CPS secretion is mediated by an ABC transporter containing KpsT and KpsM as its nucleotide-binding domain (NBD) and transmembrane domain, respectively. The transporter partners with the periplasmic and inner-membrane-anchored KpsE subunit, a class-3 polysaccharide co-polymerase (PCP), as well as with KpsD, which is assumed to form an outer-membrane pore. The KpsMT transporter is surrounded by a cage of eight KpsE subunits extending about 80 Å into the periplasm. Cryo-electron microscopy analyses of the KpsMT–KpsE complex in six different states reveal a KpsE-encaged ABC transporter, rigid-body conformational rearrangements of KpsMT during ATP hydrolysis and recognition of a glycolipid inside a membrane-exposed electropositive canyon.

We determined cryo-EM structures of the KpsMT–KpsE complex in two nucleotide-free states (Apo 1 and Apo 2), bound to ADP–AlF4− mimicking an ATP post-hydrolysis state, and in an ATP-complexed conformation after introducing the E151Q Walker B mutation into the active site of KpsT. The most complete KpsE assembly described hereafter was obtained with an ATP-bound KpsMT transporter. As expected, in the presence of ATP, the NBDs are closely associated with an Mg–ATP complex bound at each nucleotide-binding site. The architecture of the KpsM dimer in the ATP-bound state resembles the Apo 1 conformation with an open electropositive canyon. However, a notable difference exists at the cytosolic entrance to the canyon. The interface helix and the N-terminal segment of TM1 shift by about 5 Å towards TM5 of the opposing KpsM subunit, thereby narrowing the canyon. The KpsMT–KpsE complex is a dimer of two KpsMT subunits, each interacting with four KpsE subunits. Conformational transitions between nucleotide-free, ATP and ADP–AlF4−-bound KpsMT states result from rigid-body movements, with no major structural rearrangements observed within the KpsE cage.

>[2x]MIELRNLTKWYPTPHGRRYVFRNLNFRFPDDVSIGLIGRNGAGKSTLMRLLGGIEAPNEGEVVTDVSISWPVGLSGGFQGSLTARENVKFVCRIYGTSHEDMLRKVRFVEEFAEIGEHFDLPMKTYSSGMRSRVAFGLSMAFDFDYYLIDQAMAVGDAQFRAKSRAVFDSRVGQANMILVSHNMNDIKEYCDVVVLVDQGQATLYEDVEAGIAAYQGSLKKAAAKPDYKDDDDK;>[2x]MGKIHLAVSERSPRVKRSPWQIQQAVLFALFLRELKTRLGGRWLGVFWVLLEPVAHIAVMTTLFSLAHRAAMPSIEYPVFLITGLIPFFMFRGLVTRLMEAIDSNRGLFAYRQVKPIDTVIARAMLEISLQSIVYLIALGTLGWLGFHFLPVRALELAGVSAVLIMLGASLGLFFAVVTNEIPQARAIVRISLLPLYFVSGVIFPVHTIPPQYLPLLQLNPVLHLIELSRASFFPQYRVLQGINLAYPAGFALLSLFLALMLYRLRRHQLASVV;>[8x]MGKIHMKLVSRLTAKRLQWALVYLPMLVATVYFLVFSADRYVSESVITVRQTSSNAPTGGMSGAALLLAGLTPASREDTCYLQTYIHSMGLLQKLDQQLKLREHFGTPLRDPLFRLWGGTSQEWFLEYYRSRVEVLMDDICGLLTVRVQGFEPEFAQALNRAILEESERFVNELSHRMAREQGQFAEAELERATARLQEAKRQLIAFQAKHKLLDPLAQAQATGTLTAELQAALTRQEAELRNALTYLNEDSYQVKALRSQINALRQQIDEERLRATAGKNGDRINAVAAEFHDLQLQVGFAEDAYKLALAAVESARIEATRKLKSLVVVEPPVLPEIAEYPRRWYNLATLLVVCCLIYGVVSLVVATIRDHQDGSGSGSHHHHHHHHHH pmcMechanistic target of rapamycin (mTOR, also known as mammalian TOR) is an essential serine/threonine protein kinase that responds to nutrients, growth factors, and cellular energy to promote cell growth. mTOR nucleates two distinct complexes, mTORC1 and mTORC2, each characterized by specific subunits, targets, downstream signaling pathways, and functions. mTORC1 contains mTOR, regulatory-associated protein of mTOR (RAPTOR), and mammalian lethal with SEC13 protein 8 (mLST8). RAPTOR binds mTORC1 substrates, including the well-characterized substrates ribosomal protein S6 kinase 1 (S6K1) and 4E binding protein 1 (4E-BP1), through a five-amino acid motif termed TOS. RAPTOR binds the LST2 TOS sequence to present LST2 to the kinase catalytic site in mTOR for phosphorylation of LST2 S670. mTORC1-dependent phosphorylation at S670 leads to monoubiquitination and stabilization of LST2.

To characterize the binding of LST2 to mTORC1, we performed cryo-EM single-particle analysis on mTORC1 in complex with full-length LST2. Interestingly, density representing LST2 was observed only in the RAPTOR TOS-binding pocket, suggesting that mTORC1 recognizes LST2 solely through the TOS sequence. Our cryo-EM data suggest that mTORC1 recognizes LST2 exclusively through the TOS sequence and that RAPTOR binds the LST2 and 4E-BP1 TOS sequences in a highly similar manner. Next, we performed a coimmunoprecipitation experiment with purified RAPTOR and full-length LST2 (WT and F401A), to determine whether the TOS motif in full-length LST2 is exposed and accessible for binding. RAPTOR clearly bound LST2-WT whereas the binding of RAPTOR to LST2-F401A was reduced 9-fold. Binding of the full-length protein to RAPTOR revealed that substitution of the first phenylalanine in the TOS motif with an alanine (F401A) is sufficient to reduce the RAPTOR–LST2 interaction approximately 9-fold. Thus, the consensus phenylalanine in the LST2 TOS motif is critical for binding to RAPTOR, as also demonstrated previously for 4E-BP1 (19).

> HHHHHHHHHHEQKLISEEDLDYKDDDDKMESEMLQSPLLGLGEEDEADLTDWNLPLAFMKKRHCEKIEGSKSLAQSWRMKDRMKTVSVALVLCLNVGVDPPDVVKTTPCARLECWIDPLSMGPQKALETIGANLQKQYENWQPRARYKQSLDPTVDEVKKLCTSLRRNAKEERVLFHYNGHGVPRPTVNGEVWVFNKNYTQYIPLSIYDLQTWMGSPSIFVYDCSNAGLIVKSFKQFALQREQELEVAAINPNHPLAQMPLPPSMKNCIQLAACEATELLPMIPDLPADLFTSCLTTPIKIALRWFCMQKCVSLVPGVTLDLIEKIPGRLNDRRTPLGELNWIFTAITDTIAWNVLPRDLFQKLFRQDLLVASLFRNFLLAERIMRSYNCTPVSSPRLPPTYMHAMWQAWDLAVDICLSQLPTIIEEGTAFRHSPFFAEQLTAFQVWLTMGVENRNPPEQLPIVLQVLLSQVHRLRALDLLGRFLDLGPWAVSLALSVGIFPYVLKLLQSSARELRPLLVFIWAKILAVDSSCQADLVKDNGHKYFLSVLADPYMPAEHRTMTAFILAVIVNSYHTGQEACLQGNLIAICLEQLNDPHPLLRQWVAICLGRIWQNFDSARWCGVRDSAHEKLYSLLSDPIPEVRCAAVFALGTFVGNSAERTDHSTTIDHNVAMMLAQLVSDGSPMVRKELVVALSHLVVQYESNFCTVALQFIEEEKNYALPSPATTEGGSLTPVRDSPCTPRLRSVSSYGNIRAVATARSLNKSLQNLSLTEESGGAVAFSPGNLSTSSSASSTLGSPENEEHILSFETIDKMRRASSYSSLNSLIGVSFNSVYTQIWRVLLHLAADPYPEVSDVAMKVLNSIAYKATVNARPQRVLDTSSLTQSAPASPTNKGVHIHQAGGSPPASSTSSSSLTNDVAKQPVSRDLPSGRPGTTGPAGAQYTPHSHQFPRTRKMFDKGPEQTADDADDAAGHKSFISATVQTGFCDWSARYFAQPVMKIPEEHDLESQIRKEREWRFLRNSRVRRQAQQVIQKGITRLDDQIFLNRNPGVPSVVKFHPFTPCIAVADKDSICFWDWEKGEKLDYFHNGNPRYTRVTAMEYLNGQDCSLLLTATDDGAIRVWKNFADLEKNPEMVTAWQGLSDMLPTTRGAGMVVDWEQETGLLMSSGDVRIVRIWDTDREMKVQDIPTGADSCVTSLSCDSHRSLIVAGLGDGSIRVYDRRMALSECRVMTYREHTAWVVKASLQKRPDGHIVSVSVNGDVRIFDPRMPESVNVLQIVKGLTALDIHPQADLIACGSVNQFTAIYNSSGELINNIKYYDGFMGQRVGAISCLAFHPHWPHLAVGSNDYYISVYSVEKRVR;> MMNRFRKWLYKPKRSDPQLLARFYYADEELNQVAAELDSLDGRKDPQRCTLLVSQFRSCQDNVLNIINQIMDECIPQDRAPRDFCVKFPEEIRHDNLAGQLWFGAECLAAGSIIMNRELESMAMRPLAKELTRSLEDVRGALRDQALRDLNTYTEKMREALRHFDVLFAEFELSYVSAMVPVKSPREYYVQQEVIVLFCETVERALDFGYLTQDMIDDYEPALMFSIPRLAIVCGLVVYADGPLNLDRKVEDMSELFRPFHTLLRKIRDLLQTLTEEELHTLERNLCISQDVEFPIRADVQGPAALAPALSAPLPPEGPLSAKAKDPDAELACSMQYDDQELEQLSRMVHRAGDEMSSLLSPPIACQSPAHRPGAEGSPGGEASPGRPRLRSGSDEEERVFFMDDVEGTAEALARPESPAGPFGWAGSTWADPQEKGQGGPGGAAGISLPASEKEEDLSNNNLEAEGTDGASLAGTSSCSCLDSRLHLDGWEVGADDAETAEMIAHRTGGMKLSATVIFNPKSPTSLDSAVATQEAASEPVAEGMDGGPHKLSTGATNCLLHSCVCCGSCGDSREDVVERLREKCSPGGVIGASYAAGLAKASDRAPERQEEAPPPSEDASNGREPKAPTSDKCLPHTSGSQVDTASGLQGEAGVAGQQEPEARELHAGSPSAHEAPQALSGSSSSTAGSCSSDKMGPEAAPAATHAAPQATREKIRSRFHGSHDLIHRLFVCISGVADQLQTNYASDLRSILKTLFEVMATKPETDDKEKLRKVTQTLRSAALEDCALCQETLSSSELAAKTRDGDFEDPPEWVPDEACGFCTACKAPFTVIRRKHHCRSCGKIFCSRCSSHSAPLPRYGQVKPVRVCTHCYMFHVTPFYSDKAGL Speckle-type POZ protein (SPOP) is a ubiquitin ligase adaptor that binds substrate proteins and facilitates their proteasomal degradation. SPOP is composed of three domains: the meprin and tumor necrosis factor receptor-associated factor homology (MATH) substrate-interaction domain and two dimerization domains, bric à brac, tramtrack, broad complex and bric à brac, tramtrack, broad complex and C-terminal Kelch. Among the regulatory signals that control Pdx1 stability and function is a degradation pathway wherein Pdx1 associates with a ubiquitin ligase adaptor, speckle-type POZ protein (SPOP). Notably, neither SB motif in Pdx1 conforms to the established SB consensus sequence, but high-resolution structural characterization suggests that the Pdx1 SB motifs share a binding mode with other substrates.

We therefore pursued crystallography of the complex between the Pdx1 peptide (human protein residues 265–283) and SPOP-MATH. The 1.7 Å resolution cocrystal structure of Pdx1–SBM2 bound to SPOP–MATH reported here places the Pdx1 peptide in the canonical substrate-binding site and is consistent with NMR titration data. Pdx1–SBM2 also deviates from the consensus SB motif sequence, containing a Pro at site 3 instead of a Ser. As is required for other characterized SPOP substrates, Pdx1–SBM2 harbors a small aliphatic residue in consensus position 1 (P269). An approximately equal number of backbone (five) and side chain (four) H-bonds contribute to the stability of the SBM2–SPOP complex. As with Pdx1–SBM1, only two of the side chain contacts involve consensus motif positions, S272 and S273, at positions 4 and 5. The other two side chain contacts involve S268, which is N-terminal to the consensus motif and similar to extended interactions between SPOP and Pdx1–SBM1 outside the consensus motif. In Pdx1–SBM2, a proline resides in position 3, but the peptide is stabilized by H-bonding by the serine residues in positions 4 and 5. In the SBM2 complex, the distinctive internal Pro is flanked by four of the five backbone contacts, three of which are unique to SBM2. Pdx1–SBM2 binds weakly with a KD > 600 μM.

> GPGKVVKFSYMWTINNFSFCREEMGEVIKSSTFSSGANDKLKWCLRVNPKGLDEESKDYLSLYLLLVSCPKSEVRAKFKFSILNAKGEETKAMESQRAYRFVQGKDWGFKKFIRRDFLLDEANGLLPDDKLTLFCEVSVVQD;> LSASPQPSSVAPRRPQEPR>[2x]ASEKLTFKTDLEKLEREKAAQIGVAIVDPQGEIVAGHRMAQRFAMCSTFKFPLAALVFERIDSGTERGDRKLSYGPD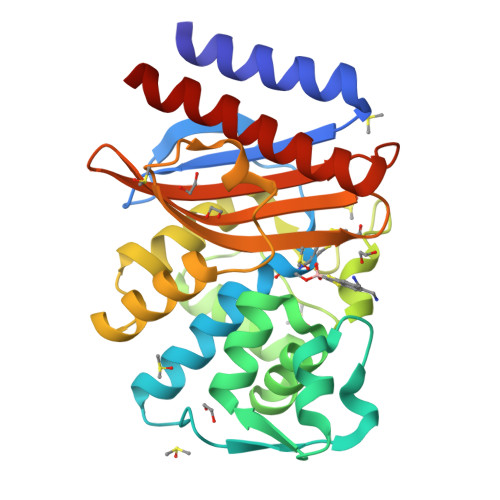MIVEWSPATERFLASGHMTVLEAAQAAVQLSDNGATNLLLREIGGPAAMTQYFRKIGDSVSRLDRKEPEMSDNTPGDLRDTTTPIAMARTVAKVLYGGALTSTSTHTIERWLIGNQTGDATLRAGFPKDWVVGEKTGTCANGGRNDIGFFKAQERDYAVAVYTTAPKLSAVERDELVASVGQVITQLILSTDK> RMNELKHAVVPIDLQSFCLEGTLALWVPALENDSEDDSEAIETADDNEKLFKKECVAYDAGVYTSNKSKGSQTLRWSIFQNRTLTIFDVSLNSKKEPLSKFNVKIHFPSNVMKDGVAFSFSEHSDTTIIYAITHARVLYYIRLSKTWFQLPDARLDDDWCLCYRPISFLNQKPDLMAAISTSEICVSFFNGGLTKIILNPKDASHYEQHIDDSSYLFSLKKYLSLQAFKADYRSPNTIISMIFLSTYNVLVMLSLDYKLKVLDLSTNQCVETIELSQTILPLQSFPYLTSDHTTNSFIALYYPDNSHGSFSIYKLNANAHSFKLNVVIEKGIIPPSLPDDEFIPWMLSDFQLISSEGSQSKFLLIIAWKSNLNTVIQKCNLSLDQDESFSCVWSHSLDSFSLIEKTFFDVPTNMSSGDISEIWLQHIFAHNTSIESIQVALLSFQNSSSQVSKNKLDKFGALTISELKNAVLSSIVSTIQIEPNSDLTGYDYYEYKRLLYNEWERFAKLVAYLDHFGDEILSINFDPSNAVTYINYANKVAFIRDPYLIESFDEEPLTKLISSLETDDPSLIEGYQILDLGRSLHSCMSFSTLSEIRYSLRELVQDLPSYSLFDTLWVFYDKHIYPNVDPDYISTLIDTLVSLENPMRDIDSLIQRLRSFDIYNHSAQSPSLFLCASVARVLDSILKKFQVSIEGFIFLLSLITSQQDYELQSKFAGCDKLFLSLLEDWRL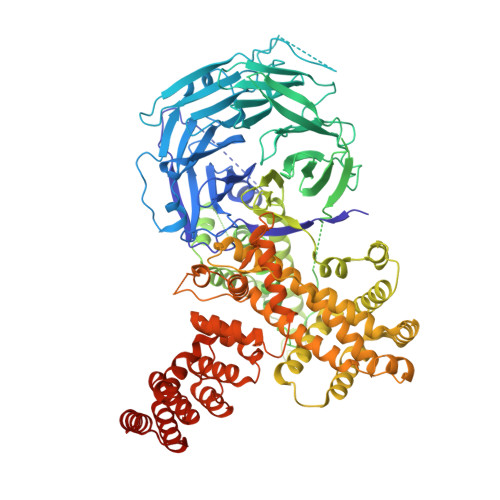VSFLLENSALLLEKFEEEDVDSTNCNLNTMEALASVNTALQFFSALNYSECFSESQISPLHATVISSLSAIFIRDDTENDLVTELVEKLFLFKQYNACMQLIGWLNSDPIAVYLKALIYLKSKEAVKAVRCFKTTSLVLYSHTSQFAVLREFQEIAEKYHHQNLLSCYYLHLSKKLFEESAYIDALEFSLLADASKETDDEDLSIAITHETLKTACAAG> EEIIWESLSVDVGSQGNPGIVEYKGVDTKTGEVLFEREPIPIGTNNMGE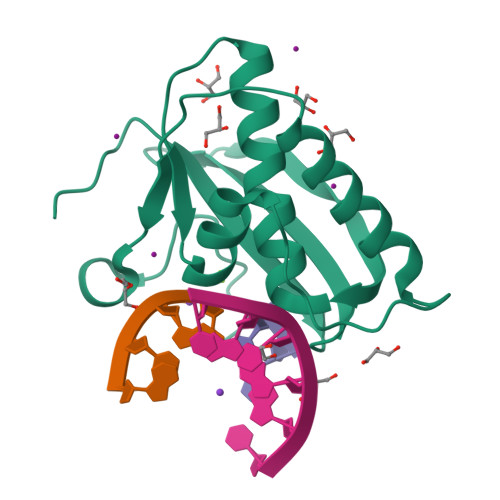FLAIVHGLRYLKERNSRKPIYSDSQTAIKWVKDKKAKSTLVRNEETALIWKLVDEAEEWLNTHTYETPILKWQTDKWGEIKADYGRK>GDNQDRTVANTQPSGPSNSTEIPALTAVETGHTSQVDPSDTIQTRHVVNFHSRSESTIENFMGRAACVFMDQYKINGEETSTDRFAVWTINIREMAQLRRKCEMFTYMRFDIEMTMVITSCQDQGTILDQDMPVLTHQIMYVPPGGPIPAKVDGYEWQTSTNPSVFWTEGNAPPRISIPFISVGNAYSSFYDGWSHFTQDGTYGYTTLNAMGKLYIRHVNRSSPHQITSTIRVYFKPKHIKAWVPRPPRLCPYINKRDVNFVVTEITDSRTSITDTPHPEHSVLATH[11x];>SPSAEECGYSDRVRSMTLGNSTITTQESANVVVGYGEWPSYLSDREATAEDQPTQPDVATCRFYTLESVQWEKTSPGWWWKFPEALKNMGLFGQNMHYHYLGRAGYTIHVQCNASKFHQGCLLVVCVPEAEMGCADTDTTFPATELTTEDTPHVFTSDSITGKKVQAAVCNAGMGVGVGNLTIFPHQWINLRTNNSATIVIPYINSVPMDNMFRHYNFTLMIIPFAPLNFTDGATAYVPITVTIAPMYAEYNGLRLAST[11x];>GVPVLNTPGSNQFLTSDDYQSPSAMPQFDETPEMHIPGEVRNLMEIAEVDSVVPVNNVTGKTKSMDAYQIPVGTGNTDKTKPIFSFQMDPGYSSVLKRTLLGEMLNYYAHWSGSVKLTFLFCGSAMATGKLLISYSPPGASVPTSRKDAMLGTHIVWDIGLQSSCVLCVPWISQSHYRMVQQDPYTSAGYITCWYQTNIVVPPGAPTSCDVLCFASACNDFSVRLLRDTPFMAQPGKLQ[11x]

Viruses from the family Picornaviridae form non-enveloped icosahedral virions that are about 30 nm in diameter. The capsid proteins VP1, VP2, VP3, and VP4 originating from a single polyprotein form a protomer, the basic building block of the icosahedral capsid. The entire capsid consists of 60 such protomers, arranged in 12 pentamer units. Here we show that the exit of the RNA from the particles of echoviruses 18 and 30 requires capsid opening and results in a loss of up to three adjacent capsid protein pentamers.

Specifically, we performed cryo-EM of echovirus 18 virions exposed to pH 6.0 for 10 min, mimicking the acidic environment that the virus encounters in endosomes. Asymmetric reconstruction combined with 3D classification identified subpopulations of echovirus 18 particles that lacked up to three pentamers of capsid protein protomers. We call the particles lacking one or several pentamers open particles. The missing pentamers always formed a single compact opening through the capsid. The absence of one pentamer of capsid protein protomers creates a 120 Å-diameter pore in the capsid. The openings formed by the removal of one or more pentamers are sufficiently large to allow release of the viral RNA, even if the genome contains double-stranded RNA segments. Reconstructions of the open particles missing one, two, or three pentamers with imposed five-fold, two-fold, and three-fold symmetries, respectively, were determined to resolutions of 3.8, 4.1, and 3.7 Å, which allowed their molecular structures to be built. Except for the missing pentamers, the open particles are similar in structure to that of the activated echovirus 18 particle: increased diameter relative to the native virus, reduced inter-pentamer contacts, absence of VP4 subunits, and holes along icosahedral two-fold symmetry axes. The capsid proteins next to the missing pentamers are more mobile than the rest of the capsid, as indicated by the three times higher temperature factors than the remainder of the capsid. Residues 1–42 from the N termini of VP1 subunits, which were previously shown to interact with membranes and facilitate enterovirus genome delivery into the cytoplasm, are not resolved in the electron density map, indicating that their structures differ among particles.>[2x]MPIAKVHRIATASPDDVSGLAAAIATGAIAPAGILAIFGKTEGNGCVNDFSRGFAVQSLQMLLRGHMGAAADEVCLVMSGGTEGGMSPHFLVFERAEGNAPEAAPALAIGRAHTPDLPFEALGRMGQVRMVAQAVRRAMAAAGITDPEDVHFVQVKCPLLTAMRVKEAEARGATTATSD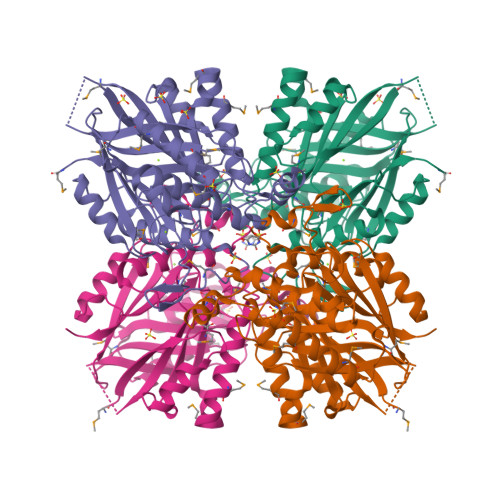TLKSMGLSRGASALGIALALGEVAEDALSDAVICADYGLWSARASCSSGIELLGHEIVVLGMSEGWSGPLAIAHGVMADAIDVTPVKAALSALGAEAGEATIVLAKAEPSRSGRIRGKRHTMLDDSDISPTRHARAFVAGALAGVVGHTEIYVSGGGEHQGPDGGGPVAVIAARTMG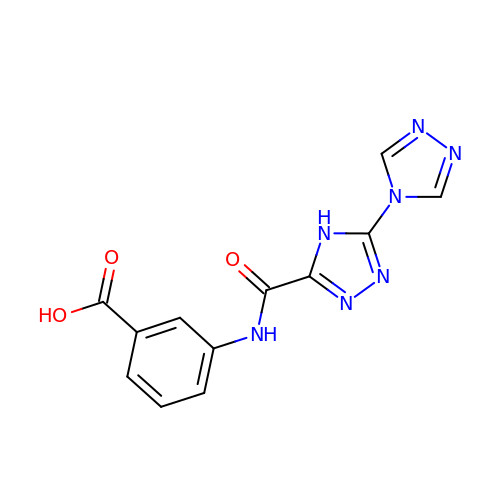3-[[5-(1,2,4-triazol-4-yl)-4H-1,2,4-triazol-3-yl]carbonylamino]benzoic acid | C12 H9 N7 O3 | JGTCMCVJBJKSBL-UHFFFAOYSA-N> MAAISVSSSPSIRCLRSACSDSSPALVSSTRVSFPAKISYLSGISSHRGDEMGKRMEGFVRSVDGKISDASFSEASSATPKSKVRKHTISVFVGDESGMINRIAGVFARRGYNIESLAVGLNRDKALFTIVVCGTERVLQQVIEQLQKLVNVLKVEDISSEPQVERELMLVKVNAHPESRAEIMWLVDTFRARVVDIAEHALTIEVTGDPGKMIAVERNLKKFQIREIVRTGKIALRREKMGATAPFWRFSAASYPDLKEQAPVSVLRSSKKGAIVPQKETSAGGDVYPVEPFFDPKVHRILDAHWGLLTDEDTSGLRSHTLS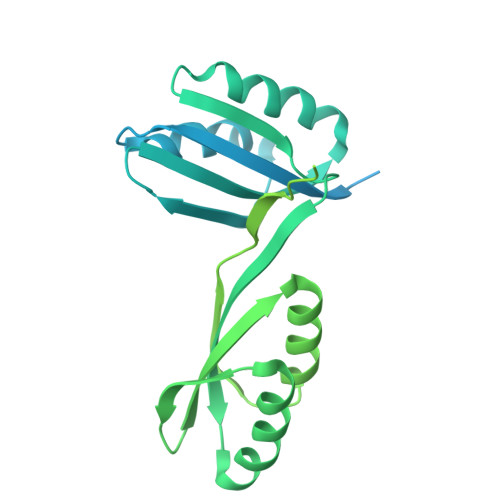LLVNDIPGVLNIVTGVFARRGYNIQSLAVGHAETKGISRITTVIPATDESVSKLVQQLYKLVDVHEVHDLTHLPFSERELMLIKIAVNAAARRDVLDIASIFRAKAVDVSDHTITLQLTGDLDKMVALQRLLEPYGICEVARTGRVALARESGVDSKYLRGYSFPLTG> DSFINIFVSIDKD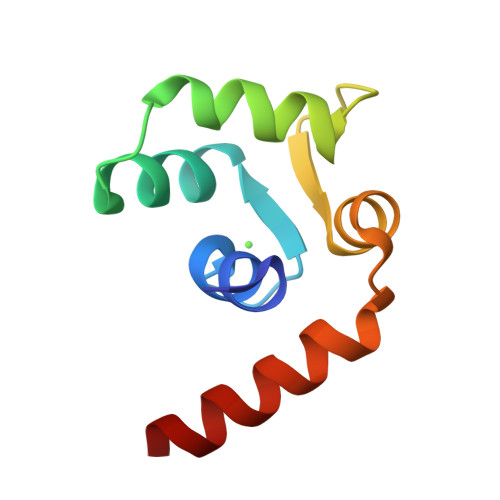GTNVISYPELEQYVAENNLDPSMVEKWKQLFDPDNTGSITLETFCSKLGLKPAEIIDFREQKGLHAA Here, we use biochemical and structural approaches to define the molecular determinants by which IstA, a transposase present in the widespread IS21 family of mobile elements, catalyzes efficient DNA transposition. The IS21 family of insertion sequences is a particularly widespread class of transposable elements. After screening several candidates, IS5376, a prototypical member of the IS21 family found in Geobacillus stearothermophilus that is highly similar to other members present in Escherichia coli, Pseudomonas aeruginosa and Yersinia pestis, was chosen for this work. By comparison, IstB is a regulatory factor and member of the AAA + (ATPases associated with various cellular activities) family of ATPases; this protein is similar to MuB and TnsC from the Mu and Tn7 mobile elements and is essential to capture the target DNA and recruit the transposase to promote efficient strand transfer.

IstA was then incubated with the optimal donor DNA in vitro (i.e., a complete pre-cleaved right transposon end with a 5 base-long 5’ overhang) and injected into a preparative gel filtration column. Despite this movement, subsequent rounds of 3D classification readily generated cryo-EM map with an estimated overall resolution of 3.4 Å. Overall, the cryo-EM structure shows that IstA self-assembles into a tetramer that engages two transposon DNA ends around a local two-fold symmetry axis. Collectively, the four transposase molecules form a highly interdigitated network in which each monomer contacts all three partner subunits. The uppermost dimers engage the TIR sequences in cis and appear to play a mostly structural function: the DDE domains in these subunits do not interact with the DNA and the catalytic triad is far (>8.5 Å) from the nucleic acid (the loop present immediately after the catalytic E233 is additionally disordered). In contrast, the lowermost dimers engage the transposon ends in trans (i.e., the DDE folds engage a different DNA end than the segment bound by their HTH elements) and appear most likely to perform a catalytic role. The DDE motifs (D124, D187 and E233) of the catalytic monomers are proximal to the signature 3’ CA dinucleotide at the end of the donor DNAs and thus are correctly positioned to perform a transposition reaction. Consistent with the known metal dependency of the catalytic reaction, extra density was observed close to the 3’-OH of the cleaved deoxyadenosine that could be modelled as a Mg2+ ion (coordinated with D124 and E233). The loop close to the catalytic glutamate (residues 225–228) that is flexible in the upper monomers becomes ordered in the catalytic subunits, where can be seen to act as a wedge that induces a base flip in the nucleotide complementary to the 3’ deoxyadenosine, which is itself stabilized by interactions with a tyrosine (Tyr 113), positioned in the loop that connects the DDE and HTH-2 domains. Notably, the division of labor of the two IstA dimers also extends to DNA recognition.

>[4x]MITRGEFFMIKEMYERGMSISDIARELGIDRKTVRKYIHSPNPPSKSKRKQRKSKLDPFKPYLQKRMLEDGVFNSEKLFFEIRQQGYTGGKTILKDYMKPFRETAKKKYTVRYETLPGEQMQVDWKEVGEVVIEGKKVKLSLFVATLGYSRMKYAVFTTSQDQEHLMECLIQSFKYFGGVPKKVLFDNMKTVTDGREQGVVKWNQRFSEFASYYGFIPKVCRPYRAQTKGKVERAIQYIMDHFYVGTAFESIEELNFLLHRWLDQVANRKPNATTGISPQERWAEESLKPLPLKDYDTSYLSYRKVHWDGSFSYKGEQWLLSAEYAGKEILVKERLNGDIRLYFRGEEISHVDQQKKVISFAEKIKKKQTEMAATISPVSVEVDTRPLSVYDAFLRGESSENLYFQ>[2x]AGSMI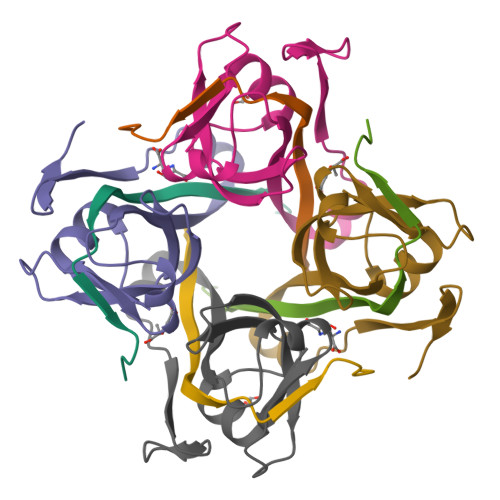RTMLQGKLHRVKVTHADLHYEG;>[2x]SCAIDQDFLDAAGILENEAIDIWNVTNGKRFSTYAIAAERGSRIISVNGAAAHCASVGDIVIIASFVTMPDEEARTWRPNVAYFEGDNEMKRTA> SERPKRVFNIYWNVPTFMCHQYDLYFDEVTNFNIKRNSKDDFQGDKIAIFYDPGEFPALLSLKDGKYKKRNGGVPQEGNITIHLQKFIENLDKIYPNRNFSGIGVIDFERWRPIFRQNWGNMKIHKNFSIDLVRNEHPTWNKKMIELEASKRFEKYARFFMEETLKLAKKTRKQADWGYYGYPYCFNMSPNNLVPECDVTAMHENDKMSWLFNNQNVLLPSVYVRQELTPDQRIGLVQGRVKEAVRISNNLKHSPKVL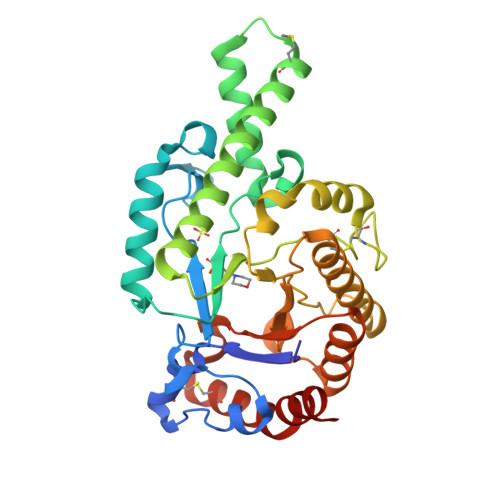SYWWYVYQDETNTFLTETDVKKTFQEIVINGGDGIIIWGSSSDVNSLSKCKRLQDYLLTVLGPIAINVTEAVN The T4 bacteriophage gp41 helicase and gp61 primase assemble into a primosome to couple DNA unwinding with RNA primer synthesis for DNA replication. The domain architecture of the gp41 helicase resembles the bacterial DnaB helicase13,14 with an NTD and a RecA-like CTD that are connected by a linking helix (LH). The gp61 primase is composed of an N-terminal ZBD and a C-terminal RPD that are linked by an 18-residue flexible loop. Here we report a series of cryo-EM structures of T4 primosome assembly intermediates.

In contrast, the other map (map 2-II at 3.4 Å resolution) showed the gp41 helicase bound to the ssDNA template that had undergone major conformational changes to become a planar ring closing the gap between subunits A and F and likely represents the active helicase configuration. In contrast, the third state of primosome assembly is represented by map 2-II at 3.4 Å resolution and map 3-II at 2.7 Å resolution. Both showed that three major conformational changes occurred when the ssDNA template-bound, open spiral of the gp41 helicase transitioned to a planar, closed-ring state. First, the N-tier rotated in plane by 60° with respect to the C-tier leading to a domain-swapped packing in the closed state, i.e. - each CTD now aligned with the neighboring NTD. Second, the linking helix (LH) from the N-tier relocated to interact with the CTD of the neighboring subunit. Finally, the N-terminal helical hairpins (enclosed in a yellow, dashed-line shape) closed in a scissor-like motion that increased their crossing angle from 100° in the open spiral form to 165° and almost antiparallel in the closed-ring form. In the active gp41 helicase, five ATPγS molecules were resolved in the C-tier with the nucleotide-binding pocket between the CTDs of subunits A and F unoccupied. In the open spiral gp41 helicase, the ssDNA binds to five (subunits B-F) of the six helicase subunits and coils inside the right-handed C-tier spiral, as compared to the activated helicase ring in which the sixth subunit (subunit A) now joins the other five subunits to coordinate the ssDNA phosphate backbone. Therefore, the 10 nt of the ssDNA stabilized in the inactive open spiral is increased to a total of 12 nt stabilized in the active closed ring gp41 helicase. Importantly, the scissor-like movement that activates the gp41 helicase exposes a hydrophobic patch on the side of the gp41 helical hairpins, which recruits the gp61 primase.

>[6x]MVEIILSHLIFDQAYFSKVWPYMDSEYFESGPAKNTFKLIKSHVNEYHSVPSINALNVALENSSFTETEYSGVKTLISKLADSPEDHSWLVKETEKYVQQRAMFNATSKIIEIQTNAELPPEKRNKKMPDVGAIPDIMRQALSISFDSYVGHDWMDDYEARWLSYMNKARKVPFKLRILNKITKGGAETGTLNVLMAGVNVGKSLGLCSLAADYLQLGHNVLYISMEMAEEVCAKRIDANMLDVSLDDIDDGHISYAEYKGKMEKWREKSTLGRLIVKQYPTGGADANTFRSLLNELKLKKNFVPTIIIVDYLGICKSCRIRVYSENSYTTVKAIAEELRALAVETETVLWTAAQVGKQAWDSSDVNMSDIAESAGLPATADFMLAVIETEELAAAEQQLIKQIKSRYGDKNKWNKFLMGVQKGNQKWVEIEQDSTPTEVNEVAGSQQIQAEQNRYQRNESTRAQLDALANELKF> QGVNIYNISAGTSVDLAAPVTTGDIVTFFSSALNLNAGAGNPNNTTLNLFAENGAYLLHIAFRLQENVIIFNSRQPDGPWLVEQAVSDVANQFAGIDGKAMVTVFDHGDKYQVVINEKTVIQYTKQISGLTSSLSYNATEETSIFSTVVEA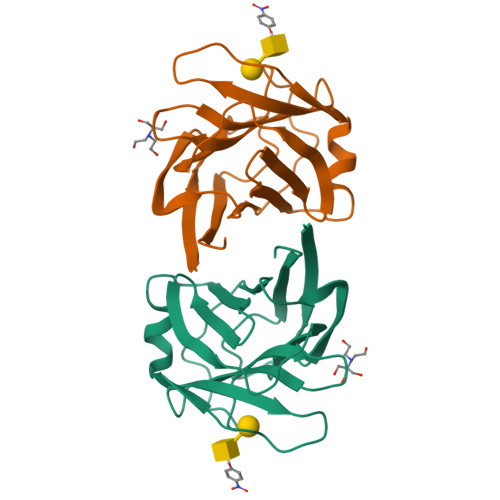VTYTGLA>[2x]GRGYEIPARLRTLHNLVIQYASQGRYEVAVPLCKQALEDLEKTSGHDHPDVATMLNILALVYRDQNKYKDAAHLLNDALAIREKTLGKDHPAVAATLNNLAVLYGKRGKYKEAEPLCKRALEIREKVLGKFHPDVAKQLSNLALLCQNQGKAEEVEYYYRRALEIYATRLGPDDPNVA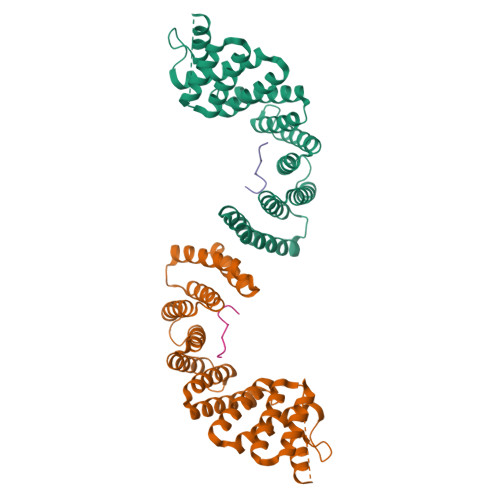KTKNNLASCYLKQGKYQDAETLYKEILTRAHEKEFGSVNGENKPIWMHAEEREESKDKRRDSAPYGEYGSWYKACKVDSPTVNTTLRSLGALYRRQGKLEAAHTLEDCASRSRKR;>NATRQLEWDDSTLSY[2x]> SDSLSFSFINFDQDERNVIAQGDARISGNNILQLTRTDSDGTPVRSTVGRILYSAQVRLWEKSTNRVANFQSQFSFFLESPLSNPADGIAFFIAPPDTAIPSGSAGGLLGLFSPKTAQNESANQVLAVEFDTFYAQNSNTWDPNYPHIGIDVNSIKSAKTVRWERREGVTLNVLVTYNPSTKTLDVVAT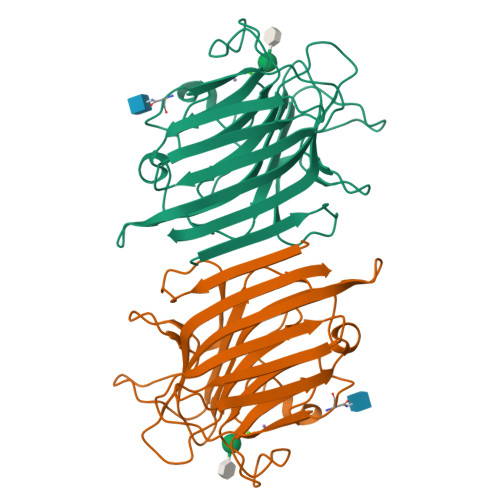YPDGQRYQISVVVDVTTVLPEWVRVGFSAASGEQFQTHNLESWSFTSTLLYTAQKE> MASRTMVSSGSEFESAVGYSRAVRIGPLVVVAGTTGSGDDIAAQTRDALRRIEIALGQAGATLADVVRTRIYVTDISRWREVGEVHAQAFGKIRPVTSMVEVTALIAPGL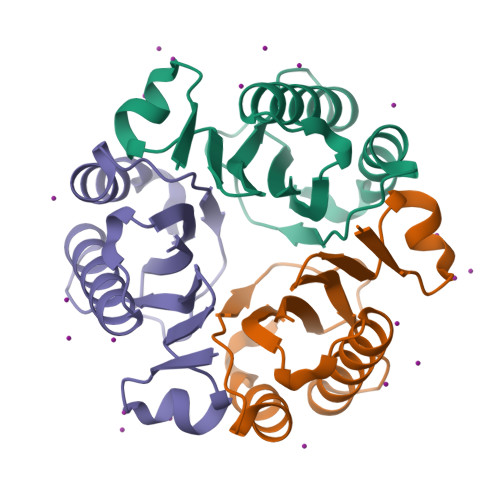LVEIEADAYVGSAVADRNSGAGPKDPSPAGGLEHHHHHH>[2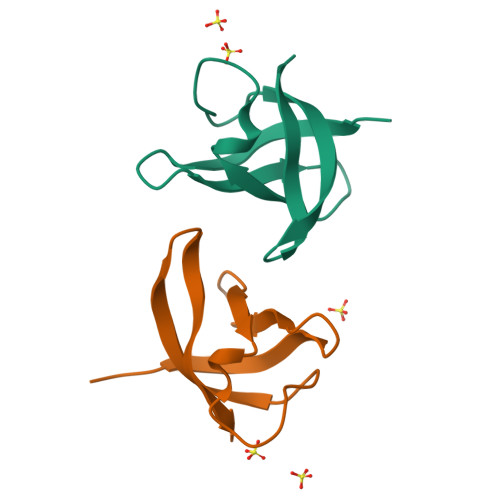x]GHMQRGKVKWFNNEKGYGFIEVEGGSDVFVHFTAIQGFKTLEEGQEVSFEIVQGNRGPQAANVVKL>APLAHCDGRGGLKLSQDMDTCEDILPCVPFSVAKSVKSLYLGRMFSGTPVIRLRFKRLQPTRLVAEFDFRTFDPEGIL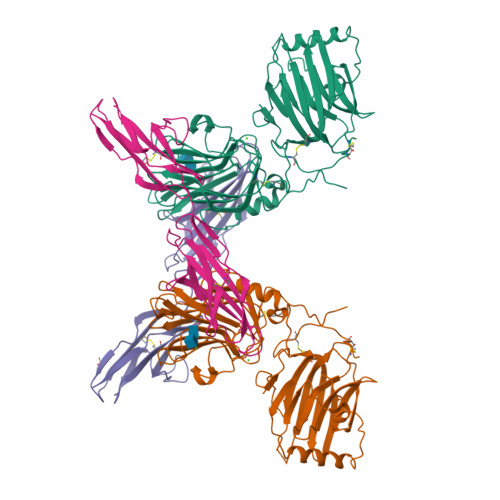LFAGGHQDSTWIVLALRAGRLELQLRYNGVGRVTSSGPVINHGMWQTISVEELARNLVIKVNRDAVMKIAVAGDLFQPERGLYHLNLTVGGIPFHEKDLVQPINPRLDGCMRSWNWLNGEDTTIQETVKVNTRMQCFSVTERGSFYPGSGFAFYSLDYMRTPLDVGTESTWEVEVVAHIRPAADTGVLFALWAPDLRAVPLSVALVDYHSTKKLKKQLVVLAVEHTALALMEIKVCDGQEHVVTVSLRDGEATLEVDGTRGQSEVSAAQLQERLAVLERHLRSPVLTFAGGLPDVPVTSAPVTAFYRGCMTLEVNRRLLDLDEAAYKHSDITAHSCPPVEPAAA[2x];>EESPFVGNPGNITGARGLTGTLRCQLQVQGEPPEVHWLRDGQILELADSTQTQVPLGEDEQDDWIVVSQLRITSLQLSDTGQYQCLVFLGHQTFVSQPGYVGLEGLPYFLEEPEDRTVAANTPFNLSCQAQGPPEPVDLLWLQDAVPLATAPGHGPQRSLHVPGLNKTSSFSCEAHNAKGVTTSRTATITVLPQQ[2x]>QVTTEAPAKVVKHSKKQDENIVVNKFKPKEPYVGRCLLNTKITG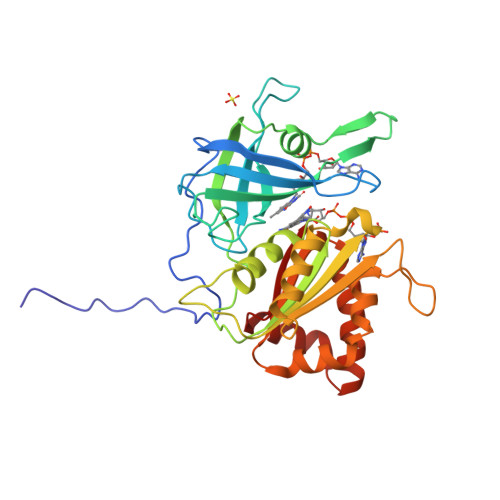DDAPGETWHMVFSTEGEVPYREGQSIGIVPDGIDKNGKPHKLRLYSIASSAIGDFGDSKTVSLCVKRLVYTNDAGEVVKGVCSNFLCDLKPGSEVKITGPVGKEMLMPKDPNATVIMLGTGTGIAPFRSFLWKMFFEKHEDYQFNGLAWLFLGVPTSSSLLYKEEFEKMKEKAPENFRLDFAVSREQVNDKGEKMYIQTRMAQYAEELWELLKKDNTFVYMCGLKGMEKGIDDIMVSLAAKDGIDWIEYKRTLKKAEQWNVEVW[2x]> MTTLLNPYFGEFGGMYVPQILMPALNQLEEAFVRAQKDPEFQAQFADLLKNYAGRPTALTKCQNITAGTRTTLYLKREDLLHGGAHKTNQVLGQALLAKRMGKSEIIAETGAGQHGVASALASALLGLKCRIYMGAKDVERQSPNVFRMRLMGAEVIPVHSGSATLKDACNEALRDWSGSYETAHYMLGTAAGPHPYPTIVREFQRMIGEETKAQILDKEGRLPDAVIACVGGGSNAIGMFADFINDTS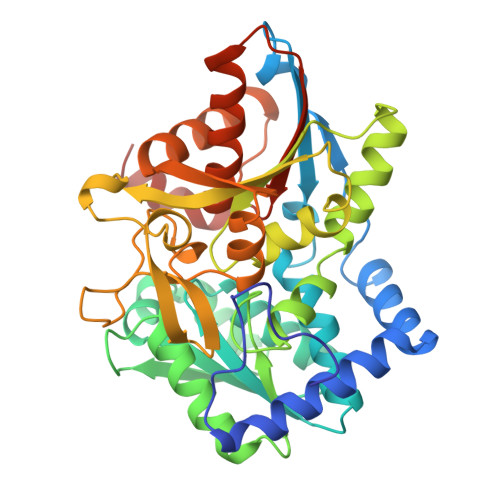VGLIGVEPGGHGIETGEHGAPLKHGRVGIYFGMKAPMMQTADGQIEESYSISAGLDFPSVGPQHAYLNSIGRADYVSITDDEALEAFKTLCRHEGIIPALESSHALAHALKMMREQPEKEQLLVVNLSGRGDKDIFTVHDILKARGLI>GHMFEKIRKILADIEDSQNEIEMLLKLAN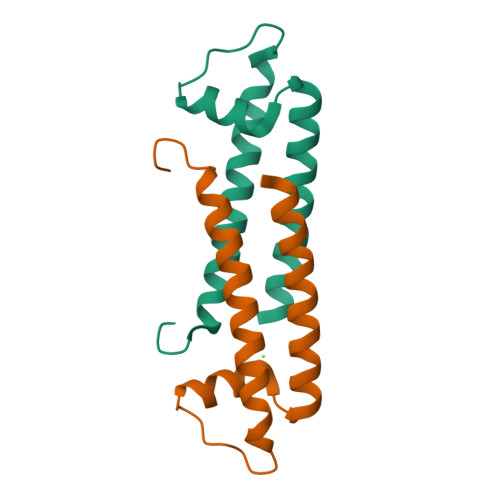LSLGDFIEIKRGSMDMPKGVNEAFFTQLSEEVERLKELINALNKIKKGLLVFGS[6x]> STVTLPETLLFVSTLDGSLHAVSKRTGSIKWTLKEDPVLQVPTHVEEPAFLPDPNDGSLYTLGSKNNEGLTKLPFTIPELVCASPSRSSDGILYMGKKQDIWYVIDLLTGEKQQTLSSAFADSLSPSTSLLYLGR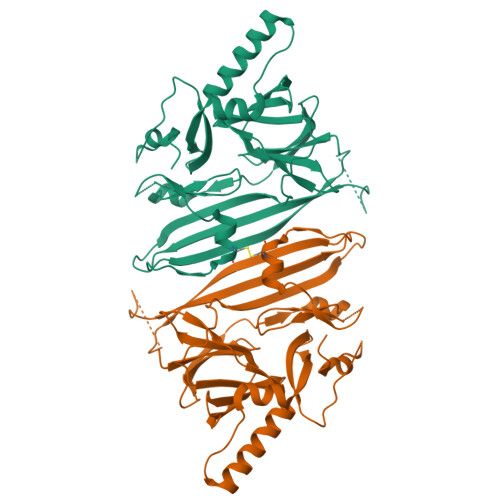TEYTITMYDTKTRELRWNATYFDYAASLPEDDVDYKMSHFVSNGDGLVVTVDSESGDVLWIQNYASPVVAFYVWQREGLRKVMHINVAVETLRYLTFMSGEVGRITKWKYPFPKETEAKSKLTPTLYVGKYSTSLYASPSMVHEGVAVVPRGSTLPLLEGPQTDGVTIGDKGESVITPSTDVKFDPGLKSKNKLNYLRNYWLLIGHHETPLSASTKMLERFPNNLPKHRENV>[4x]HMCDSALTAQANDLRIYQVMVESFVNGDDAIGHGTGYGTSHHKGDLQGIIDSLDYIESLGMNAIWLTPIFDSIPVEGQDHWADRLDATGYFTSNYFAVDPRFGTMEQAKELVEKAHEKGLYVFFDGVFGHHKDNVVPSPEGRLPVGENNPVSYPESLAFYQEVATFWIEELKIDGWRLDQAYQVPTEAWTAIRASVDEASKSVTYVNSKGEAVNPLGYMVAQIWNNENYIKETGYGAEGEPALCSAFDFPVRYRVVETFAANENGIGNKGGKWLDEGMNLHRLYPSHAQPNLMLGNHDLVRFGDLLQRGNIASPEQAEYWERHKAALSFQAAYSGPITLYYGEEIGDELEGYAQKVEQDCAVQGLCDDHVARTSANIDGLTVNLNEKQRDLKQYVSQLMTLRAAHPALSRGERTNIVANETVYIDHKQADDDALIYMVSTTADQDTVELKASDIASDGQLVDLLTGKVHSAINGEYQISLAPFEAKFLLIETPSASGLTKVATVSAASSLIGEGFMAQCDNPTIEGDGPIGKTLYVVGDFADASWKQKPHRAYRYVGENTYQAVVDEKAGAFRMQYASKDWSPQFTADGLELTPGKTASLKRGGYGQDTAVTLPEAGQYVWSLKFTDSGDPEQIMVSKCP

The GH13_37 subfamily is the most recently established α-amylase subfamily. It was created on the basis of the isolation and phylogenetic analysis of a novel α-amylase, designated AmyP, from a marine metagenomic library. AmyP exhibits high substrate specificity for starch over pullulan or cyclomaltodextrins, efficiently hydrolyzing starch into glucose, maltose and maltotriose. AmyP is a raw-starch-degrading enzyme (RSDE), thus making it of potential interest in the food processing and green-fuels communities. The AmyPΔSBD is composed of A, B, and C domains and shares structural features with other GH13 α-amylases.

Substitution of the glutamic acid at position 221 of AmyP with glutamine (E221Q mutation) resulted in nearly complete inactivation of the enzyme. The E221Q mutant displayed 0.125% of the activity of the wild-type (WT) enzyme in thses assays. The crystal structure of the E221Q catalytic domain mutant AmyPΔSBD in complex with maltotriose was obtained through co-crystallization of the E221Q mutant of full-length AmyP with γ-cyclodextrin (γ-CD) (AmyP-E221Q/γ-CD). This structure was determined to a resolution of 2.55 Å by molecular replacement by using the crystal structure of the Bacillus stearothermophilus TRS40 neopullulanase (pdb accession code 1J0H27) as a search model. Peptide sequencing of protein bands from the dissolved crystal sample by sodium dodecyl sulfate polyacrylamide gel electrophoresis (SDS-PAGE) and liquid chromatography-mass spectrometry (LC-MS) showed that partial degradation of the SBD domain of the AmyP-E221Q/γ-CD crystals had occurred. The structure of AmyP-E221Q/γ-CD contains electron density representing a maltotriose molecule bound to the active site and occupying subsites -1, -2 and -3, whereas the structure of AmyP/β-CD contains electron density representing a maltose molecule at subsites -2 and -3. These observations suggested that the E221Q mutant possesses activity for γ-CD and the WT enzyme possesses activity for β-CD at the high concentration in the crystallization drop, thus producing maltotriose from γ-CD and maltose from β-CD, respectively. Stick superposition of the active site of AmyPΔSBD-E221Q complexed with maltotriose on the structures of GTA and TASKA indicated the remainder of the strictly conserved residues for subsites −1 and −2, including residues participating in hydrogen bonding and aromatic stacking interactions. Interestingly, the -3 subsite of AmyPΔSBD, which is formed by the hydrogen-bond-forming residues Tyr36, Asp367 and His368, is novel. In this work, the resulting glucan in the crystal structures, however, was not the cyclodextrin, but a degradation product, G2 in the case of the WT enzyme and G3 in the case of the active-site mutant.>[12x]GMQENTRLRIAIQKSGRLSKESIELLSECGVKMHIHEQSLIAFSTNLPIDILRVRDDDIPGLIFDGVVDLGIIGENVLEENELERQ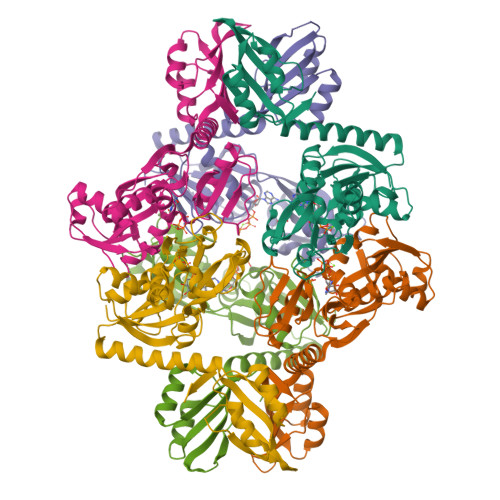SLGENPSYKLLKKLDFGYCRLSLALPQENKFQNLKDFEGLRIATSYPQLLKRFMKENGINYKNCTLTGSVEVAPRANLADAICDLVSSGATLQANNLKEVKVIYESRACLIQKENALSKEKQALVDKIMLRVAGVMQARESKYIMLHAPKEKLDKIQALLPGVERPTILPLAHDEKNVALHMVSKENLFWETMEALKEEGASSILVLPIEKMLK>[4x]MLKLLDNWDSVTSTFSKLREQLGPVTQEFWDNLEKETEGLRQEMSKDLEEVKAKVQPYLDDFQKKWQEEMELYRQKVEPLRAELQEGARQKLHELQEKLSPLGEEMRDRARAHVDALRTHLA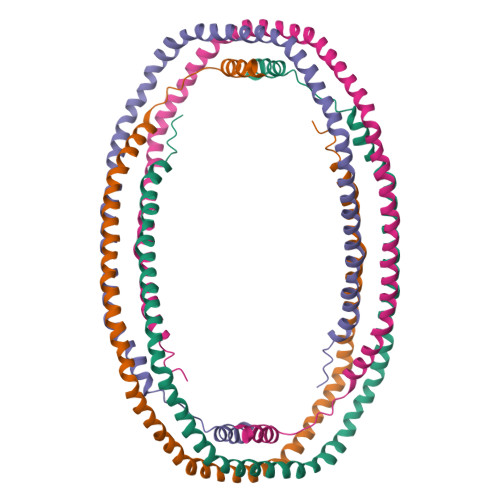PYSDELRQRLAARLEALKENGGARLAEYHAKATEHLSTLSEKAKPALEDLRQGLLPVLESFKVSFLSALEEYTKKLNTQ5-azanyl-6-ethyl-1H-pyrimidine-2,4-dione | C6 H9 N3 O2 | 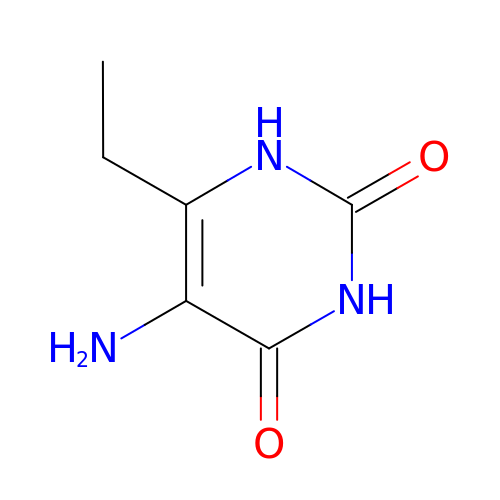NHAGBFNQWVFUGY-UHFFFAOYSA-N~{N}-[3-[methyl(7~{H}-pyrrolo[2,3-d]pyrimidin-4-yl)amino]cyclobutyl]methanesulfonamide 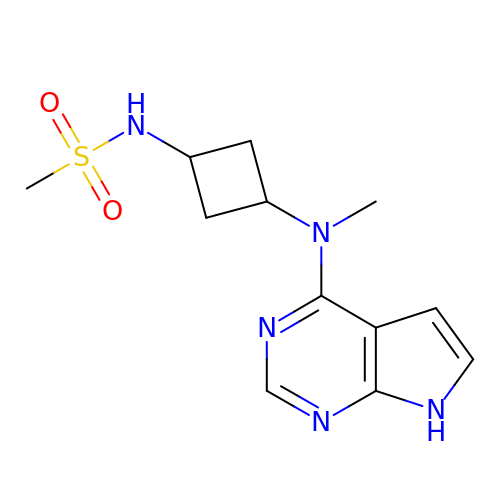| C12 H17 N5 O2 S | QZOGHNDWZHFIJP-DTORHVGOSA-N>GSHMGGVDVLAAVPLSEETEFKVELFVKPVIGNAEG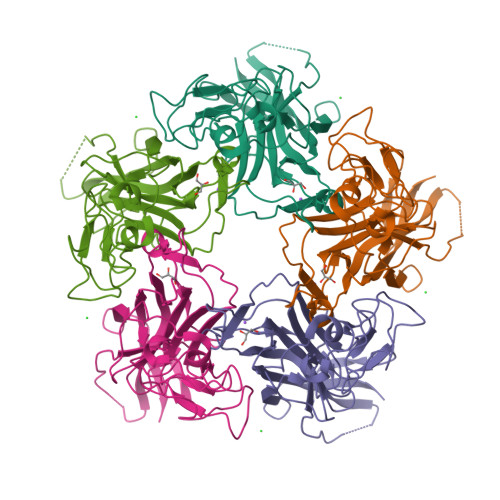TTPHYWSISSPLKTAEAANVTPDADTTVCYSLSQVAPPDIPNQVSECDMLIWELYRMETEVLVLPVLNAGILTTGGVGGIAGPQLYFWAVGGQPLDVLGLAPTEKYKGPAQYTVNPKTNGTVPHVYSSSETPKARVTNEKYSIESWVADPSRNDNCRYFGRMVGGAATPPVVSFSNNSTIPLLDENGIGILCLQGRLYITCADLLGVNKNRVHTGLSRFFRLHFRQRRVRN[5x]> MADIEDTHFETGDSGASATFPMQCSALRKNGFVMLKGRPCKIVEMSTSKTGKHGHAKVHLVGIDIFNGKKYEDICPSTHNMDVPHVKREDYQLTDISDDG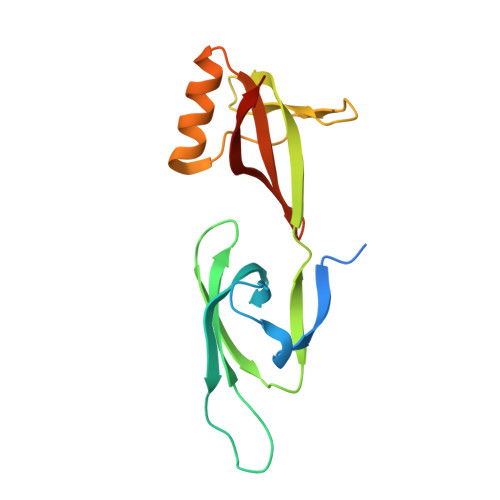YLTLMADNGDLREDLKIPDGDLGTQLRSDFDSGKELLCTVLKSCGEECVIAVKANTALDK> MYG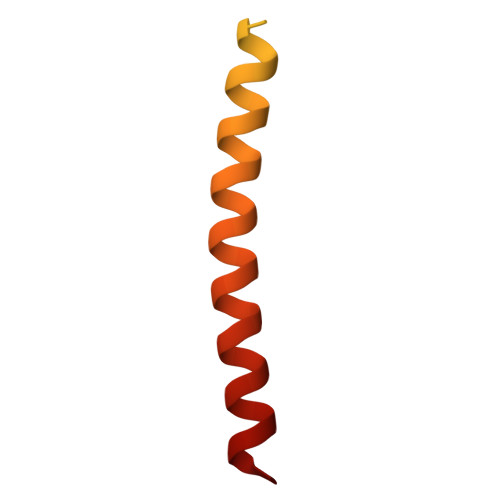KIIFVLLLSEIVSISALSTTEVAMHTSTSSSVTKSYISSQTNGETGQLVHRFTVPAPVVIILIILCVMAGIIGTILLISYSIRRLIKA> LERLVGPQDATHCSPGLSCRLWDSDILCLPGDIVPAPGPVLAPTHLQTELVLRCQKETDCDLCLRVAVHLAVHGHWEEPEDEEKFGGAADSGVEEPRQASLQAQVVLSFQAYPTARCVLLEVQVPAALVQFGQSVGSVVYDCFEAALGSEVRIWSYTQPRYEKELQHTQQLPDCRGLEVWNSIPSCWALPWLQVSADGDNVHLVLQVSEEQHFGLSLYWNQVQGPPKPRWHKNLTGPQIITLQHTDLVPCLCIQVWPLEPDSVRTNICPFREDPRAHQNLWQAARLRLLTLQSWLLDAPCSLPAEAALCWRAPGGDPCQPLVPPLSWEQV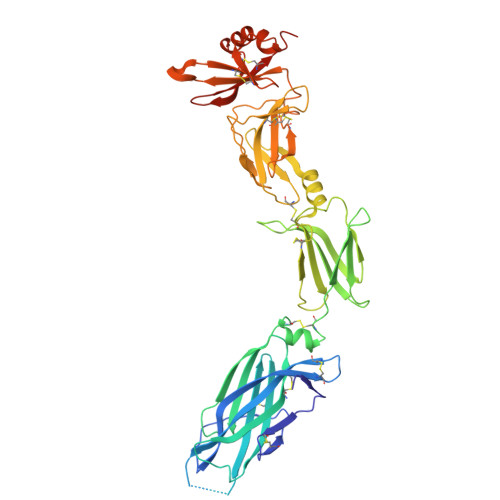TVDKVLEFPLLKGHPNLCVQVQSSEKLQLQECLWADSLGPLKDDVLLLETRGPQDQRSLCALEPSGCTSLPSKASTRAARLGEYLLQDLQSGQCLQLWDDDLGALWACPMDKYIHKREFRH> PPGVDCPMEFWTKEENQSVVVDFLLPTGVYLNFPVSRNANLSTIKQLLWHRAQYEPLFHMLSGPEAYVFTCINQTAEQQELEDEQRRLCDVQPFLPVLRLVAREGDRVKKLINSQISLLIGKGLHEFDSLCDPEVNDFRAKMCQFCEEAAARRQQLGWEAWLQYSFPLQLEPSAQTWGPGTLRLPNRALLVNVKFEGSEESFTFQVSTKDVPLALMACALRKKATVFRQPLVEQPEDYTLQVNGRHEYLYGSYPLCQFQYICSCLHSGLTPHLTMVHSSSILAMRDEQSNPAPQVQKPRAKPPPIPAKKPSSVSLWSLEQPFRIELIQGSKVNADERMKLVVQAGLFHGNEMLCKTVSSSEVSVCSEPVWKQRLEFDINICDLPRMARLCFALYAVIEKAKKARSTKKKSKKADCPIAWANLMLFDYKDQLKTGERCLYMWPSVPDEKGELLNPTGTVRSNPNTDSAAALLICLPEVAPHPVYYPALEKILELGRHSECVHVTEEEQLQLREILERRGSGELYEHEKDLVWKLRHEVQEHFPEALARLLLVTKWNKHEDVAQMLYLLCSWPELPVLSALELLDFSFPDCHVGSFAIKSLRKLTDDELFQYLLQLVQVLKYESYLDCELTKFLLDRALANRKIGHFLFWHLRSEMHVPSVALRFGLILEAYCRGSTHHMKVLMKQGEALSKLKALNDFVKLSSQKTPKPQTKELMHLCMRQEAYLEALSHLQSPLDPSTLLAEVCVEQCTFMDSKMKPLWIMYSNEEAGSGGSVGIIFKNGDDLRQDMLTLQMIQLMDVLWKQEGLDLRMTPYGCLPTGDRTGLIEVVLRSDTIANIQLNKSNMAATAAFNKDALLNWLKSKNPGEALDRAIEEFTLSCAGYCVATYVLGIGDRHSDNIMIRESGQLFHIDFGHFLGNFKTKFGINRERVPFILTYDFVHVIQQGKTNNSEKFERFRGYCERAYTILRRHGLLFLHLFALMRAAGLPELSCSKDIQ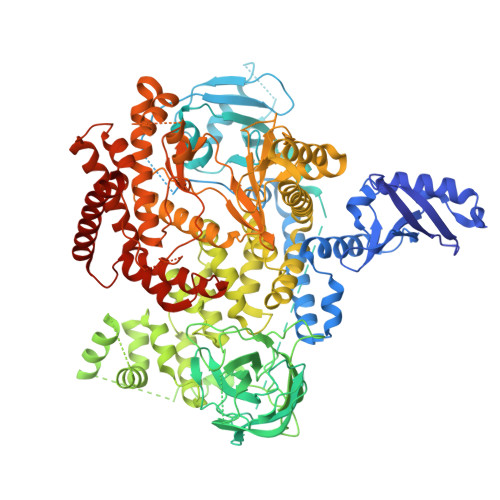YLKDSLALGKTEEEALKHFRVKFNEALRESWKTKVNWLAHNVSKDNRQ> VLGGHECQPHSQPWQAALF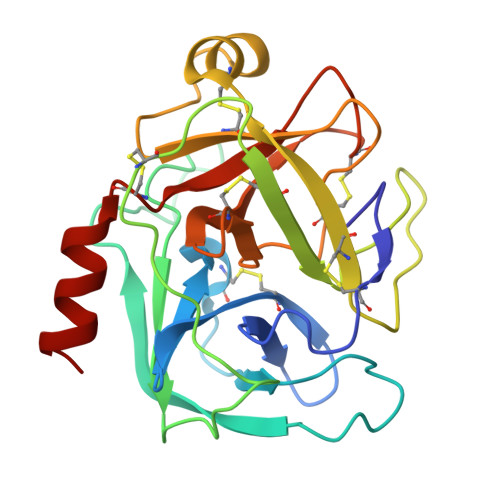QGQQLLCGGVLVGGNWVLTAAHCKKPKYTVRLGDHSLQNKDGPEQEIPVVQSIPHPCYNSSDVEDHNHDLMLLQLRDQASLGSKVKPISLADHCTQPGQKCTVSGWGTVTSPRENFPDTLNCAEVKIFPQKKCEDAYPGQITDGMVCAGSSKGADTCQGDSGGPLVCDGALQGITSWGSDPCGRSDKPGVYTNICRYLDWIKKIIGSKG>MSLSVAIIGPGAVGTT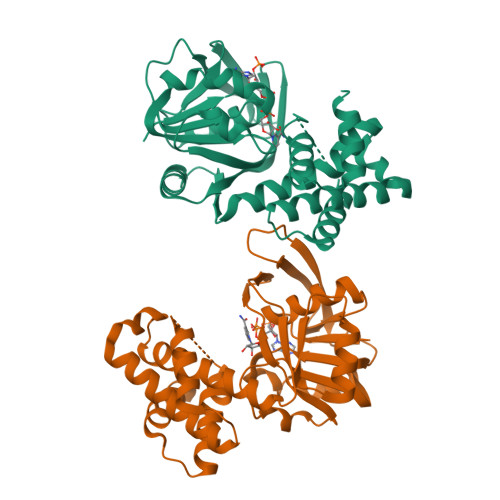IAYELQQSLPHTTLIGRHAKTITYYTVPHAPAQDIVVKGYEDVTNTFDVIIIAVKTHQLDAVIPHLTYLAHEDTLIILAQNGYGQLEHIPFKNVCQAVVYISGQKKGDVVTHFRDYQLRIQDNALTRQFRDLVQDSQIDIVLEANIQQAIWYKLLVNLGINSITLLGRQTVAIMHNPEIRILCRQLLLDGCRVAQAEGLNFSEQTVDTIMTIYQGYPDEMGTSMYYDIVHQQPLEVEAIQGFIYRRAREHNLDTPYLDTIYSFLRAYQQNEGHHHHHH[2x]In contrast, budding yeast chromosomes have point centromeres with single nucleosomes that are defined by conserved ~125 nucleotide segments, including three centromere determining elements (CDEs): CDEI (8 bp), CDEII (~80–90 bp, and AT-rich), and CDEIII (~25 bp). In budding yeast, the centromere CBF3 complex guides the deposition of CENP-A, an H3 variant, to form the centromeric nucleosome in a DNA sequence-dependent manner. CBF3 is a four-protein complex consisting of subunits Ndc10, Skp1, Ctf3, and two copies of Cep3. Here, we determine the structures of the centromeric nucleosome containing the native CEN3 DNA and the CBF3core bound to the canonical nucleosome containing an engineered CEN3 DNA.

We were able to observe intact particles of the CBF3core bound to the CEN3-601 H3 nucleosome and obtained the cryo-EM density map at 4.2 Å resolution. It allowed us to build the structural models that showed multiple conformations for the major core region of the CBF3core. The major core region of the CBF3core showing multiple conformations is connected to the Gal4 domain through a flexible linker and moves as a rigid body (relative to the Gal4-nucleosome region). Examination of the available structures of the CBF3core in the free and DNA-bound forms shows that the major core regions have the same structure but display different orientations relative to the Gal4 domain. In some of the conformations, the Ctf3 subunit is close to the α2 helix of H2B and the L1 loop of H3. We found that the Cbf13 subunit was close to the five charged residues of the α2 helix of H2B and the three residues in loop 1 of CENP-ACse4. The model suggests potential formation of a salt bridge between Ctf13 K282 and H2B E117 and hydrophobic interactions between Cft13 P297 and CENP-ACse4 K1987. We mutated the residues in the α2 helix of H2B to Ala, deleted the three residues in loop 1 of CENP-ACse4, and measured the binding affinities of CBF3core to the nucleosomes containing the histone mutants. Each of the two mutants showed little effects on the binding affinity, and when combined, they decreased the binding affinity by only less than a factor of two. These results showed that CBF3core only made weak and dynamic contacts with the core histones.

> MGPSFNPVRFLELPIDIRKEVYFHLDGNFCGAHPYPIDILYKSNDVELPGKPSYKRSKRSKKLLRYMYPVFATYLNIFEYSPQLIEKWLEYAFWLRYDCLVLDCFKVNHLYDGTLIDALEWTYLDNELRLAYFNKASMLEVWYTFKEYKKWVIDSVAFDELDLLNVSNIQFNIDNLTPQLVDKCLSILEQKDLFATIGEVQFGQDEEVGEEKDVDVSGANSDENSSPSSTIKNKKRSASKRSHSDNGNVGATHNQLTSISVIRTIRSMESMKSLRKITVRGEKLYELLINFHGFRDNPGKTISYIVKRRINEIRLSRMNQISRTGLADFTRWDNLQKLVLSRVAYIDLNSIVFPKNFKSLTMKRVSKIKWWNIEENILKELKVDKRTFKSLYIKEDDSKFTKFFNLRHTRIKELDKSEINQITYLRCQAIVWLSFRTLNHIKLQNVSEVFNNIIVPRALFDSKRVEIYRCEKISQVLVIGSRSGSENLYFQGSKRRWKKNFIAVSAANRFKKISSSGAL;>[2x]MFNRTTQLKSKHPCSVCTRRKVKCDRMIPCGNCRKRGQDSECMKSTKLITASSSKEYLPDLLLFWQNYEYWITNIGLYKTKQRDLTRTPANLDTDTEECMFWMNYLQKDQSFQLMNFAMENLGALYFGSIGDISELYLRVEQYWDRRADKNHSVDGKYWDALIWSVFTMCIYYMPVEKLAEIFSVYPLHEYLGSNKRLNWEDGMQLVMCQNFARCSLFQLKQCDFMAHPDIRLVQAYLILATTTFPYDEPLLANSLLTQCIHTFKNFHVDDFRPLLNDDPVESIAKVTLGRIFYRLCGCDYLQSGPRKPIALHTEVSSLLQHAAYLQDLPNVDVYREENSTEVLYWKIISLDRDLDQYLNKSSKPPLKTLDAIRRELDIFQYKVDSLEEDFRSNNSRFQKFIALFQISTVSWKLFKMYLIYYDTADSLLKVIHYSKVIISLIVNNFHAKSEFFNRHPMVMQTITRVVSFISFYQIFVESAAVKQLLVDLTELTANLPTIFGSKLDKLVYLTERLSKLKLLWDKVQLLDSGDSFYHPVFKILQNDIKIIELKNDEMFSLIKGLGSLVPLNKLRQESLLEEEDENNTEPSDFRTIVEEFQSEYNISDILSGSGGSGENLYFQ;> MVTSNVVLVSGEGERFTVDKKIAERSLLLKNYLNDMHDSNLQNNSDSESDSDSETNHKSKDNNNGDDDDEDDDEIVMPVPNVRSSVLQKVIEWAEHHRDSNFPDEDDDDSRKSAPVDSWDREFLKVDQEMLYEIILAANYLNIKPLLDAGCKVVAEMIRGRSPEEIRRTFNIVNDFTPEEEAAIRRENEWAEDR>MDYTVGTYLAERLVQIGLKHHFAVAGDYNLVLLDNLLDNKNMEQVYCCNELNCGFSAEGYARAKGAAAAVVTYSVGALSAFDAIGGAYAENLPVILISGAPNNNDHAAAHVLHHALGKTDYHYQLEMAKNITAAAEAIYTPEEAPAKIDHVIKTALREKKPVYLEIACNIASMPCAAPGPASALFNDEASDEASLNAAVEETLKFIENRDKVAVLVGSKLRAAAAEEAAVKFADALGGAVATMAAAKSFFPEENPHYIGTSWGEVSYPGVEKTMKEADAVIALAPVFNDYSTTGWTDIPDPKKLVLAEPRSVVVNGIRFPSVHLKDYLTRLAEKVSKKTGALDFFKSLNAGELKKADPADPSAPLVNAEIARQIEDLLTPNTTVIAETGDSWFNAQRMKLPNGARVEYEMQWGHIGWSVPAAFGYAVGAPERRNILMVGDGSFQLTAQEVAQMVRLKLPVIIFLINNYGYTIEVMIHDGPYNNIKNWDYAALMEVFNGNGGYDSGAGKGLKAKTAAELEEAIKVALDNTDGPTLIECFIAREDCTEELVKW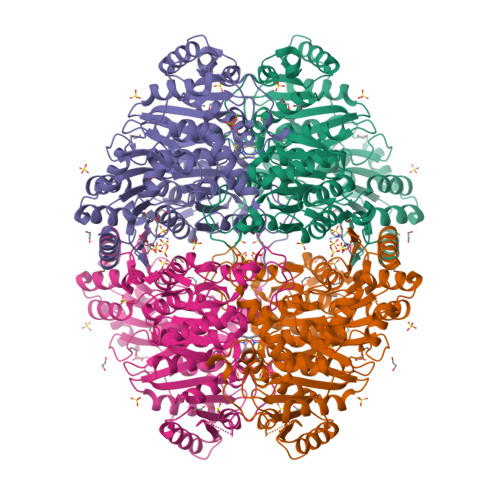GERVAAANSRKPVNKLLLEHHHHHH[2x]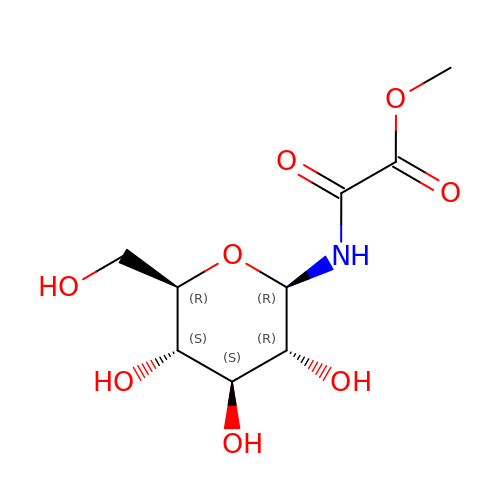N-[methoxy(oxo)acetyl]-beta-D-glucopyranosylamine | C9 H15 N O8 | OHCAXSUQOPLGLU-QOHYDMMQSA-N2-CHLORO-9-(2-DEOXY-2-FLUORO-B -D-ARABINOFURANOSYL)-9H-PURIN-6-AMINE | C10 H11 Cl F N5 O3 | 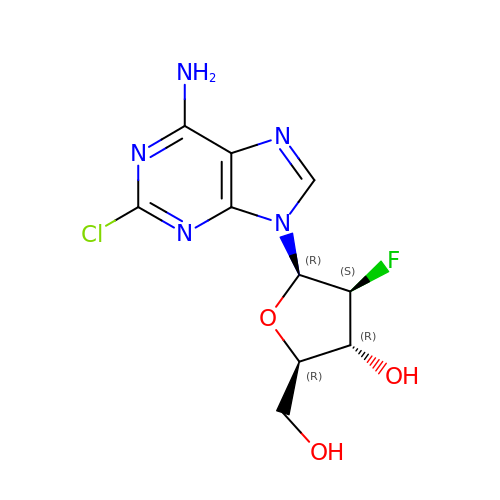WDDPHFBMKLOVOX-AYQXTPAHSA-N> MSSVEELTQLFSQVGFEDKKVKEIVKNKKVSDSLYKLIKETPSDYQWNKSTRALVHNLASFVKGTDLPKSELIVNGIINGDLKTSLQVDAAFKYVKANGEASTKMGMNENSGVGIEITEDQVRNYVMQYIQENKERILTERYKLVPGIFADVKNLKELKWADPRSFKPIIDQEVLKLLGPKDERDLIKKKTKNNEKKKTNSAKKSSDNSASSGPKRTMFNEGFLGDLHKVGENPQAYPELMKEHLEVTGGKVRTRFPPEPNGYLHIGHSKAIMVNFGYAKYHNGTCYLRFDDTNPEKEAPEYFESIKRMVSWLGFKPWKITYSSDYFDELYRLAEVLIKNGKAYVCHCTAEEIKRGRGIKEDGTPGGERYACKHRDQSIEQNLQEFRDMRDGKYKPGEAILRMKQDLNSPSPQMWDLIAYRVLNAPHPRTGTKWRIYPTYDFTHCLVDSMENITHSLCTTEFYLSRESYEWLCDQVHVFRPAQREYGRLNITGTVLSKRKIAQLVDEKFVRGWDDPRLFTLEAIRRRGVPPGAILSFINTLGVTTSTTNIQVVRFESAVRKYLEDTTPRLMFVLDPVEVVVDNLSDDYEELATIPYRPGTPEFGERTVPFTNKFYIERSDFSENVDDKEFFRLTPNQPVGLIKVSHTVSFKSLEKDEAGKIIRIHVNYDNKVEEGSKPKKPKTYIQWVPISSKYNSPLRVTETRVYNQLFKSENPSSHPEGFLKDINPESEVVYKESVMEHNFGDVVKNSPWVVDSVKNSEFYVEEDKDS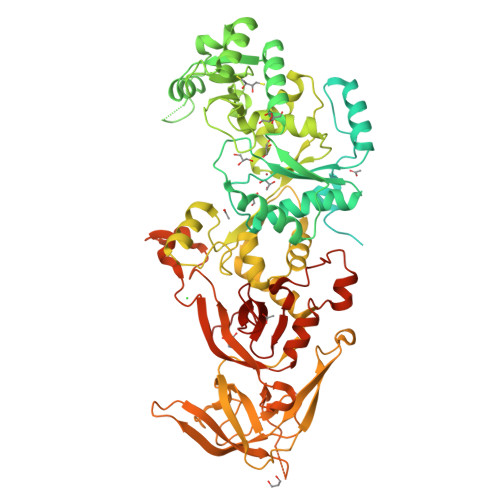KEVCRFQAMRVGYFTLDKESTTSKVILNRIVSLKDATSKSGLEALFQ>[3x]AQVQQLTPAQQAALRNQQAMAANLQARQIVLQQSYPVIQQVETQTFDPANRSVFDVTPANVGIVKGFLVKVTAAITNNHATEAVALTDFGPANLVQRVIYYDPDNQRHTETSGWHLHFVNTA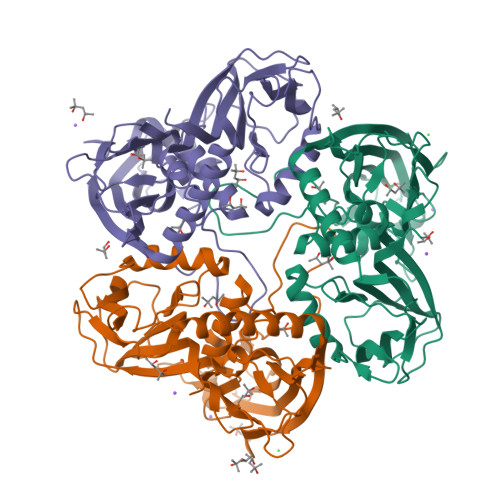KQGAPFLSSMVTDSPIKYGDVMNVIDAPATIAAGATGELTMYYWVPLAYSETDLTGAVLANVPQSKQRLKLEFANNNTAFAAVGANPLEAIYQGAGAADCEFEEISYTVYQSYLDQLPVGQNGYILPLIDLSTLYNLENSAQAGLTPNVDFVVQYANLYRYLSTIAVFDNGGSFNAGTDINYLSQRTANFSDTRKLDPKTWAAQTRRRIATDFPKGVYYCDNRDKPIYTLQYGNVGFVVNPKTVNQNARLLMGYEYFTSRTELVNAGTISTT>[2x]ALETLAFDGRTYIEYLNAVIESELTNEIPAEKALQSNHFELSLRTEATQGLVLWIGKAAERADYMALAIVDGHLQLSYDLGSQPVVLRSTVKVNTNRWLRIRAHREHREGSLQVGNEAPVTGSSPLGATQLDTDGALWLGGLQKLPVGQALPKAYGTGFVGCLRDVVVGHRQLHLLEDAVTKPELRPCPTP;>VNECAEEGYCSQGCTNSEGAFQCWCEAGYELRPDRRSCKALGPEPVLLFANRIDIRQVLPHRSEYTLLLNNLENAIALDFHHRRELVFWSDVTLDRILRANLNGSNVEEVVSTGLESPGGLAVDWVHDKLYWTDSGTSRIEVANLDGAHRKVLLWQSLEKPRAIALHPMEGTIYWTDWGNTPRIEASSMDGSGRRIIADTHLFWPNGLTIDYAGRRMYWVD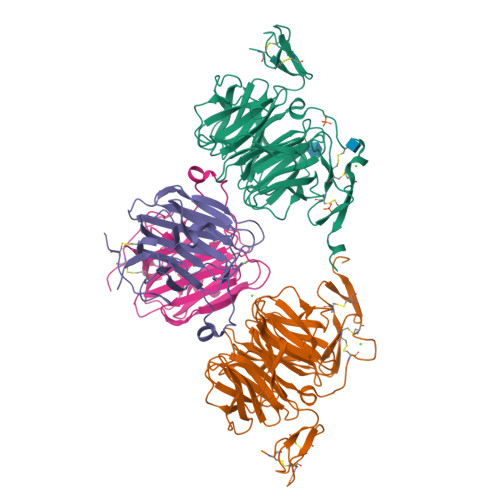AKHHVIERANLDGSHRKAVISQGLPHPFAITVFEDSLYWTDWHTKSINSANKFTGKNQEIIRNKLHFPMDIHTLHPQRQPAGKNRCGDNNGGCTHLCLPSGQNYTCACPTGFRKINSHACALEVLFQG[2x]>MDNSHDSDSVFLYHIPCDNCGSSDGNSLFSDGHTFCYVCEKWTAGNEDTKERASKRKPSGGKPMTYNVWNFGESNGRYSALTARGISKETCQKAGYWIAKVDGVMYQVADYRDQNGNIVSQKVRDKDKNFKTTGSHKSDALFGKHLWNGGKKIVVTEGEIDMLTVMELQDCKYPVVSLGHGASAAKKTCAANYEYFDQFEQIILMFDMDEAGRKAVEEAAQVLPAGKVRVAVLPCKDANECHLNGHDREIMEQVWNAGPWIPDGVVSALSLRERIREHLSSEESVGLLFSGCTGINDKTLGARGGEVIMVTSGSGMGKSTFVRQQALQWGTAMGKKVGLAMLQESVEETAEDLIGLHNRVRLRQSDSLKREIIENGKFDQWFDELFGNDTFHLYDSFAEAETDRLLAKLAYMRSGLGCDVIILDHISIVVSASGESDERKMIDNLMTKLKGFAKSTGVVLVVICHLKNPDKGKAHEEGRPVSITDLRGSGALRQLSDTIIALERNQQGDMPNLVLVRILKCRFTGDTGIAGYMEYNKETGWLEPSSYSGEEESHSESTDWSNDTDF[6x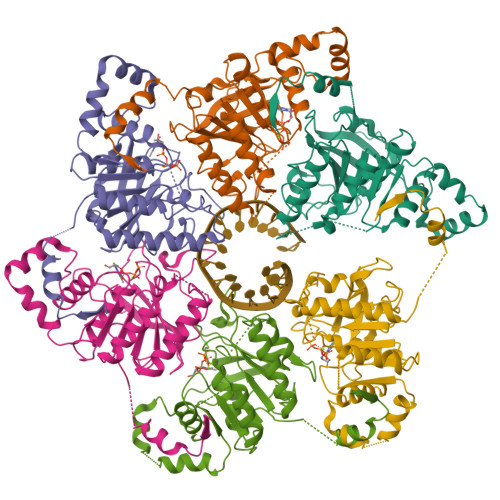]Dispatched (Disp) is a 12-transmembrane protein that plays a critical role in the Hedgehog (Hh) signaling pathway by releasing the dually lipidated ligand HhN from the membrane, a prerequisite step to the downstream signaling cascade. Structural studies have revealed common features of RND transporters. They typically contain a membrane-embedded domain splitting into two pseudosymmetrical halves with six transmembrane helices (TMHs) each and two extracellular domains that are associated with the two transmembrane halves. In this study, we report the characterization, expression, purification, and cryo-EM structure determination of Disp from Hypsibius dujardini, a type of water bear.

The ones with higher yields were then combined. This yielded the construct (dubbed wbDisp*) that consists of residues (1–111, 123–530, 542–1116). To determine its 3D structure, wbDisp* purified in digitonin was subjected to cryo-EM analysis. A 6.5-Å map was reconstructed using 62,850 particles, showing a slingshot shape with the two extracellular blobs as the branches and the transmembrane helices as the handle. To obtain a model at this low resolution, the recently published structure of the fruit fly homolog (ffDisp) was trimmed to poly-alanine and fit into the map, followed by manual mutation and adjustments. WBDisp showed a monomeric structure with 12 transmembrane helices. It contains two pseudosymmetrical repeats with each repeat containing six TMHs and a soluble domain. The two slingshot braches create a wide opening with a gap of ∼21 Å at the bottom and of ∼32 Å at the top, enough to accommodate an HhN molecule which has a dimension of ∼20 × 30 × 38 Å. The water bear Disp (wbDisp) has an overall similar structure with ffDisp and hDisp, despite that they only share modest sequence homology. By contrast, noticeable differences, particularly at the transmembrane domain, were observed between the wbDisp* and the published structures. Specifically, the inner leaflet part of TMH1, TMH3, and TMH6 shift towards TMH2, compressing the membrane core region, and this is repeated for the TMH1’, TMH3’, TMH6’, and TMH2’ in the C-terminal pseudosymmetrical half.

> MGSHHHHHHHHHHHHGSPRQLVRRRKKTVMQRYAHFLAHHPFLILTLTFCANIVLLLVIVCTDSLPAFDDPQAGFEPRGSLINQRAQAWRNFLERDGVVQPSTRRKATTTKPVAARQNAPVQEIGTGLRNSTVKENVFSSSGMASLGPITQPRGFFCSRPLLGHAKLILRRKDAGNLLNLEGIRELCQLDADIRRLDEFQSCSEESADTGRLCRTWNLPNYVAVLAGKTSCHQLEEHDIRNVLNLTATCLPFYRSGQLKADCSTSEDDGKTMQEDTITCPGVPTDCIKDSSIYHLLYFISDKESRETGYSSMKHTLAVLPVWSSPAALPLYRALQWGNFTRPDDDGPIQVIGMEMGLGDRLFNTALLEDTLYVGVAAGVVVVVLWLYTGSLFVTLMNLMAIFFSLVVSYFLYVFVFRLTFFPFMNLLTCVIIVAIGADALVIFARLWHLAKTEKDDGRFEKVVHATFRHAAQAILVSSLTASAALFSDIVNPIIAIRCFSIFAGLTVLVHLFFAVTWMPACFVVADKWGSSVYVCTKSPVCRLLYRCRCLHSGLRQYCDYFRIFFEKLLPCLVIRLKWMWMASFVLLTVGACVVVFVFPGLQLASGRTFSLWNSGHPSEQYRLLKDRFAFEENRNLNNNEKVSLHFVWGVLALNQAALLDPTDTGITTMDGRFNMSDPLSQIWMLKFCADLRQQTFFDNSTQSDNACYFDSFMLWMETGACSGHSQFPYPPATFIRCVHTFSNSFPQAKHFGPNFNSLHQIDSFVLRLQTSQLFSHSYTAMQQLHQHVDQWFTAALRTAPPSLQGAWFTGDFAFFDLQQSLISGTALSLIVSLFVAFLVLFFTTLNVGVSLIAITVIAGIMLATTAALVLMEWQLSVFESTIIGLAIGLSVDFTLHYAVSYCCAESYEERELKTNIVISEMASCVTMSAVTTFLAGALMIPSDILFYRQLGLFIITVTAISLLYATIFLPACLAVLGPQGAFLQFHYPSCRPLCCRPDPSKLVEKSMHSSAEFDTTYTTGGTYDHHRETKQCFHQSINQPYQGKALRSPSAAANNHHVVVISATPEQPPKTHPALLLDVDPDLADEETDSVGELGSVPTSRGPSRGTSLIGTLEVLFQ> GPKVQTDPPSVPICDLYPNGVFPKGQECEYPPTQDGRTAAWRTTSEEKKALDQASEEIWNDFREAAEAHRQVRKYVMSWIKPGMTMIEICEKLEDCSRKLIKENGLNAGLAFPTGCSLNNCAAHYTPNAGDTTVLQYDDICKIDFGTHISGRIIDCAFTVTFNPKYDTLLKAVKDATNTGIKCAGID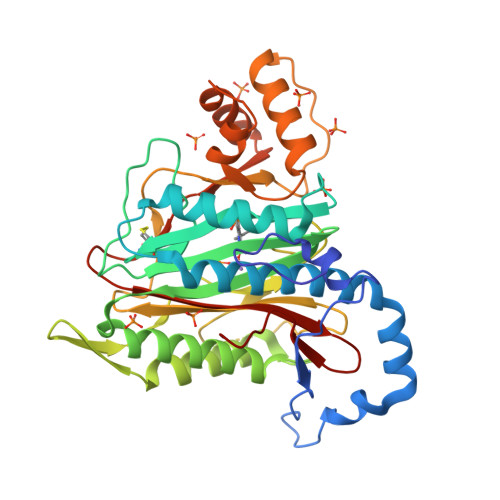VRLCDVGEAIQEVMESYEVEIDGKTYQVKPIRNLNGHSIGQYRIHAGKTVPIVKGGEATRMEEGEVYAIETFGSTGKGVVHDDMECSHYMKNFDVGHVPIRLPRTKHLLNVINENFGTLAFCRRWLDRLGESKYLMALKNLCDLGIVDPYPPLCDIKGSYTAQFEHTILLRPTCKEVVSRGDDY> XLR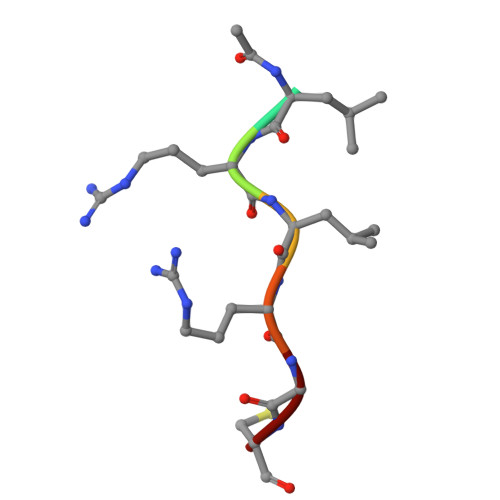LRGC>[8x]MSFPGWGPYPPVERDETSAITYSSKLHGSVTVRDPYSQLEVPFEDSEETKAFVHSQRKFARTYLDENPDREAWLETLKKSWNYRRFSALKPESDGHYYFEYNDGLQSQLSLYRVRMGEEDTVLTESGPGGELFFNPNLLSLDGNAALTGFVMSPCGNYWAYGVSEHGSDWMSIYVRKTSSPHLPSQERGKDPGRMNDKIRHVRFFIVSWTSDSKGFFYSRYPPEDDEGKGNAPAMNCMVYYHRIGEDQESDVLVHEDPEHPFWISSVQLTPSGRYILFAASRDASHTQLVKIADLHENDIGTNMKWKNLHDPWEARFTIVGDEGSKIYFMTNLKAKNYKVATFDANHPDEGLTTLIAEDPNAFLVSASIHAQDKLLLVYLRNASHEIHIRDLTTGKPLGRIFEDLLGQFMVSGRRQDNDIFVLFSSFLSPGTVYRYTFGEEKGYRSL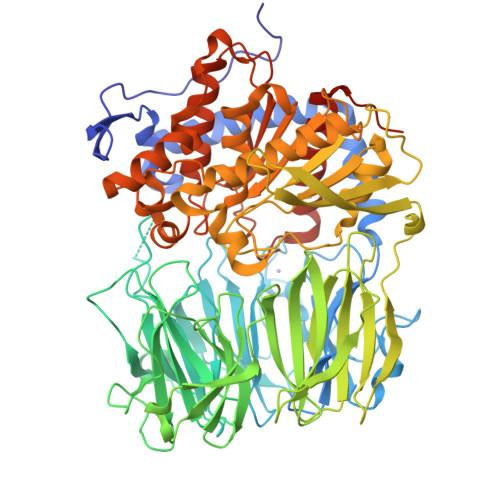FRAISIPGLNLDDFMTESVFYPSKDGTSVHMFITRPKDVLLDGTSPVLQYGYGGFSLAMLPTFSLSTLLFCKIYRAIYAIPNIRGGSEYGESWHREGMLDKKQNVFDDFNAATEWLIANKYASKDRIAIRGGANGGVLTTACANQAPGLYRCVITIEGIIDMLRFPKFTFGASWRSEYGDPEDPEDFDFIFKYSPYHNIPPPGDTVMPAMLFFTAAYDDRVSPLHTFKHVAALQHNFPKGPNPCLMRIDLNSGHFAGKSTQEMLEETADEYSFIGKSMGLTMQTQGSVDSSRWSCVTV>[2x]SNAGNEVAKAQQA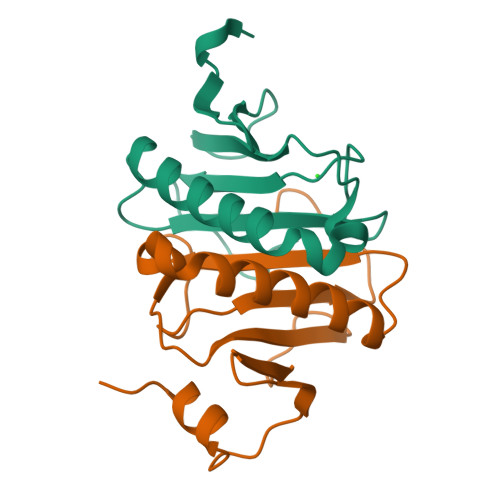TPGGAAPTIFSRILDKSLPADILYEDQQCLVFRDVAPQAPVHFLVIPKKPIPRISQAEEEDQQLLGHLLLVAKQTAKAEGLGDGYRLVINDGKLGAQSVYHLHIHVLGGRQLQWPPG>[2x]SMNYFVGNSLGVNLTGIEKAIINRLNLFKEMGRPAQCVFLSWNRYLYRNAQNYITSSDYINMYDFFQEATYLERNEPFDWLSYWTDECHYTLKHVENSHDFRIYDQERFLMYAHFQDPKYRILDYVNHFDSQRRKVKRDFYDVRGFLSCSRILVDKQQTLCEFFYNPEGDTKLEKYFSYKDGKPEVQKIIVYYANKQYFFNNETELGAFFIKQLYQHGDLFFSDRNVYTAPIFNLTPESIPVVAVLHSTHIKNIDALDSSPFKNVYKAMFENLSRYRAIIVSTEQQKLDVEKRINHTIPVVNIPVGYSETIDTPVQTLDQRSVKLISVARYSPEKQLHQQIELIKRLVSYVPKIELHMYGFGSESKKLNELIQKYGLENHVYLRGFLSNLDQEYSDAYLSLITSNMEGFSLALLESLAHGVPVISYDIKYGPNELITSDFNGYLITKNDEDALFDKVKYVIDHPEVQQRLSKGSLAKAQQYSKASLIKQWDQFVRLILEHHHHH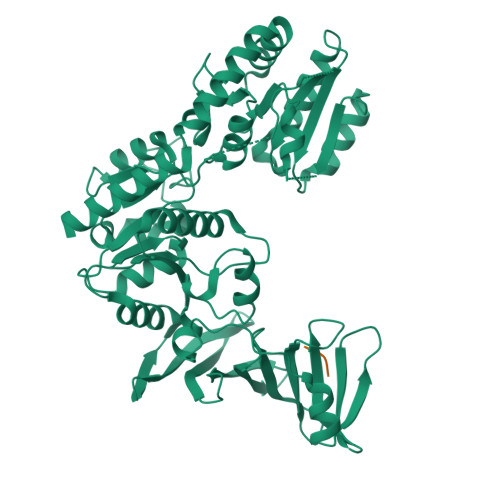H;> DSD> IIGGTESKPHSRPYMAYLEIVTSNGPSKFCGGFLIRRNFVLTAAHCAGRSITVTLGAHNITEEEDTWQKLEVIKQFRHPKYNTSTLHHDIMLLKLKEKASLTLAVGTLPFPSQFNFVPPGRMCRVAGWGRTGVLKPGSDT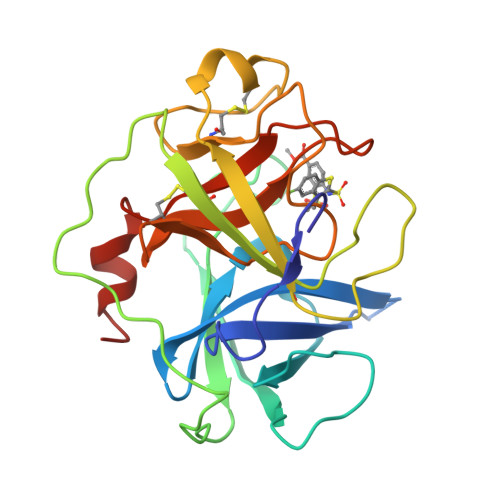LQEVKLRLMDPQACSHFRDFDHNLQLCVGNPRKTKSAFKGDSGGPLLCAGVAQGIVSYGRSDAKPPAVFTRISHYRPWINQILQAN>MHHHHHHDPPCEELEIVWKNIKAEARALADCEPMLASFYHATLLKHENLGSALSYMLANKLASPIMPAIAIREVVEEAYAADPEMIASAACDIQAVRTRDPAVDKYSTPLLYLKGFHALQAYRIGHWLWNKGRRALAIFLQNQVSVSFQVDIHPAAKIGRGIMLDHATGIVVGETAVIEDDVSILQSVTLGGTGKTSGDRHPKIREGVMIGAGAKILGNIEVGRGAKIGAGSVVLQPVPPHTTAAGVPARIVGKPGSDKPSMDMDQHFNGIHHTFEYGDG[2x]

Serine O-acetyltransferase (CysE) is an enzyme in many bacteria that catalyzes the first step in l-cysteine biosynthesis by transferring an acetyl group from acetyl coenzyme A (acetyl-CoA) to l-serine to form O-acetylserine. Lack of the CysE/CysK-dependent l-cysteine biosynthesis pathway in mammals suggests that those bacterial enzymes may become targets for antimicrobial agents. In this study, we used recombinant CysE cloned from Salmonella Typhimurium (StCysE). Here, we demonstrated that alkyl gallates such as octyl gallate (OGA) could act as potent CysE inhibitors in vitro and in bacteria.

We determined the crystal structure of a complex of StCysE and CoA. Two subunits of the StCysE-CoA complex were in an asymmetric unit: one subunit formed a trimer that was related to a crystallographic three-fold axis, and the other subunit also formed a trimer that was related to the same crystallographic three-fold axis; together they formed a hexamer (B: residues: 1–245). The CoA molecule bound to a hydrophobic crevice located between β-helices at three equidistant active site locations related to a three-fold axis near a cysteine-binding site. The di-phosphate portion of CoA interacted with the side chain of Lys-187 via electrostatic interaction and formed a hydrogen bond to the side chain of Thr-235. The pantothenic group of CoA interacted with the main chain of Thr-185 and Ala-222. The adenine group of CoA was fit in the hydrophobic pocket of the StCysE. There was no electron density in the C-terminal region of StCysE (residues: 245-C-terminus), so the hydrophobic region of StCysE was exposed to the solvent.>GSHMIEVVCNDRLGKKVRVKCNTDDTIGDLKKLIAAQTGTRWNKIVLKKWYTIFKDHVSLGDYEIHDGMNLELYYQ[6x];>SLSIEETNKLRAKLGL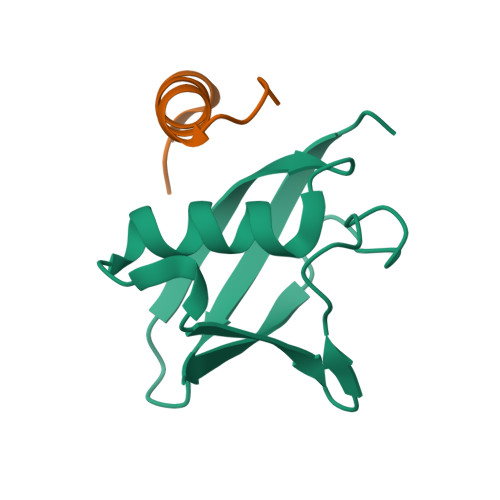KPL[6x]>[2x]PGQGDVQTPNPSVTPTQTPIPTISGNALRDYAEARGIKIGTCVNYPFYNNSDPTYNSILQREFSMVVCENEMKFDALQPRQNVFDFSKGDQLLAFAERNGMQMRG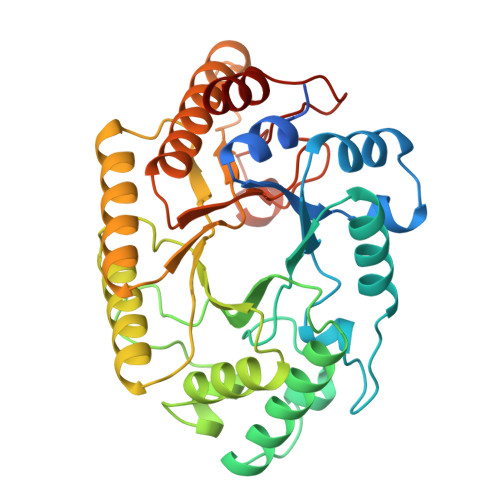HTLIWHNQNPSWLTNGNWNRDSLLAVMKNHITTVMTHYKGKIVEWDVANECMDDSGNGLRSSIWRNVIGQDYLDYAFRYAREADPDALLFYNDYNIEDLGPKSNAVFNMIKSMKERGVPIDGVGFQCHFINGMSPEYLASIDQNIKRYAEIGVIVSFTEIDIRIPQSENPATAFQVQANNYKELMKICLANPNCNTFVMWGFTDKYTWIPGTFPGYGNPLIYDSNYNPKPAYNAIKEALMGY> GGHLIDRHVGKTEAELLNRVSTGNVKSASSFTDRTTAEAVTSKAIDSNQAKIDSYLSGSQKGYLEIDYQSNVPIGISVSRGSTNVSSVTNARIIIARDPSMPT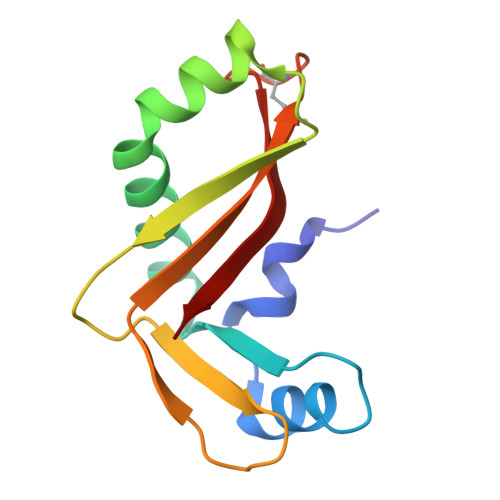GYKIITGYPTP> ATVPDLESDSFHVDWYSTYAELRETAPVTPVRFLGQDAWLVTGYDEAKAALSDLRLSSDPKKKYPGVEVEFPAYLGFPEDVRNYFATNMGTSDPPTHTR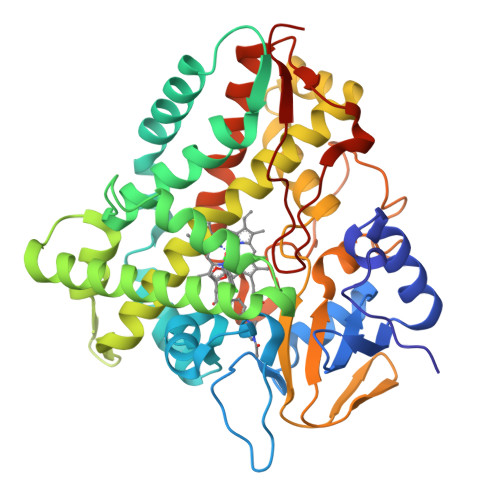LRKLVSQEFTVRRVEAMRPRVEQITAELLDEVGDSGVVDIVDRFAHPLPIKVICELLGVDEAARGAFGRWSSEILVMDPERAEQRGQAAREVVNFILDLVERRRTEPGDDLLSALISVQDDDDGRLSADELTSIALVLLLAGFEASVSLIGIGTYLLLTHPDQLALVRADPSALPNAVEEILRYIAPPETTTRFAAEEVEIGGVAIPQYSTVLVANGAANRDPSQFPDPHRFDVTRDTRGHLSFGQGIHFCMGRPLAKLEGEVALRALFGRFPALSLGIDADDVVWRRSLLLRGIDHLPVRLDG> PSDKPVAHVVANPQAEGQLQWSNRRANALLANGVELRDNQLVVPIEGLFLIYSQVLFKGQGCPSTHVLLTHTISRIAVSYQTKV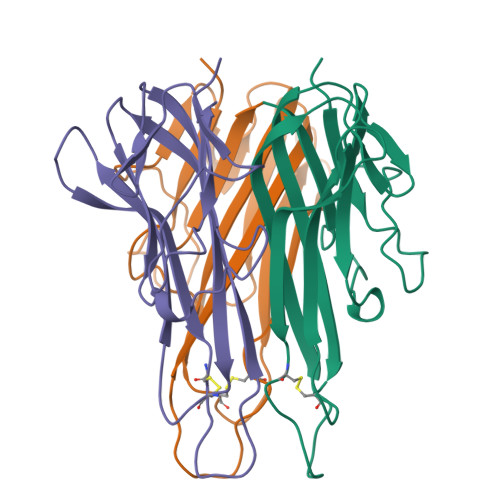NLLSAIKSPCQRETPEGAEAKPWYEPIYLGGVFQLEKGDRLSAEINRPDYLDFAESGQVYFGIIAL> MVEKIGDVEGFKVIDNGEPTADIVVGSTAAAADVVSAANVAAKVGSMMFKEGEGGSDAKAPVAFKAPLAVLDTEVSLDAANKKLILVGGPVANALTKELADAGKIEMTVESPATLAVVAGAAN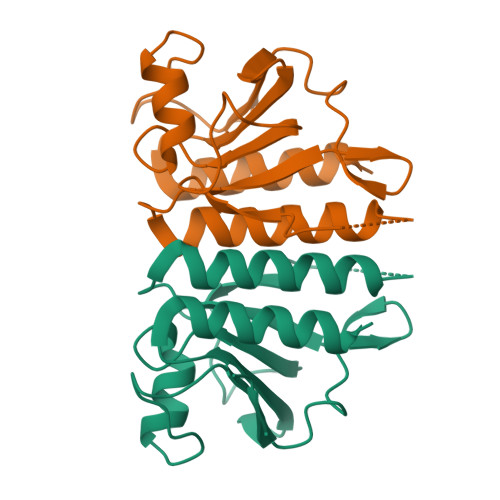GNDVLVVAGGDRAATAEAANALIEMLLEHHHHHH> MGNAVVVKKDFRIDLENELFIRGEVTLVEDQIKKPVLVISHGFRGYKDWGFWPYVAAWFAERGFYVVHFDFSRVGALNSGADEASVQKLSTVSRELSDLDAILSNLREHRLPLAEQAETERISLLGHARAGGSNIIFAAEHSYIGSVIAWNGGPPPKAAAGNPNPFINDDVEH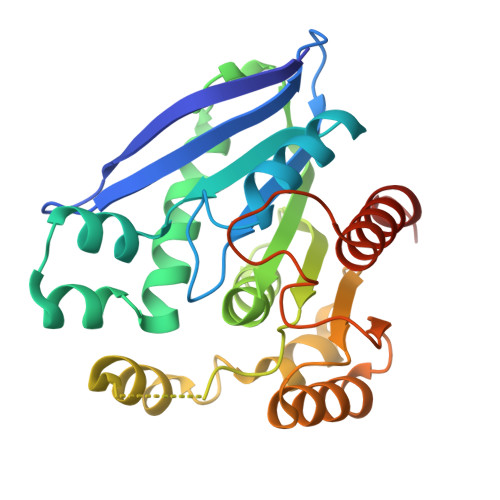NKQRFDTARLLASLTAPVLIIQGGKDREALLEGQQLLKEAAPNQTYISIPDADHSFGGEHPFHHTTPYLEEALEVTHSFITKHYLEHHHHHH> QSLVADVGDDHHAWHRLLDQALNQRRFELFFQPVVAAQDTQLVLHYKVLSRLLDEQGQTIPAGRFLPWLERFGWTARLDRLMLERV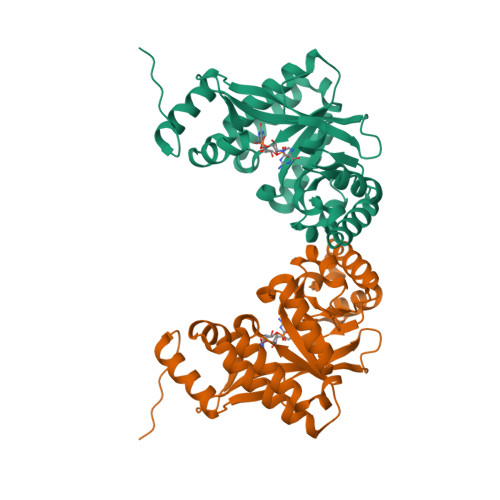LEQMAGHEESLALNLSSATLADPQALNKVFEILRAHSNLGARLTLEIGEEQLPEQAVLEQLTRRLRELGFSLSLQRFGGRFSMIGNLARLGLAYLKIDGSYIRAIDQESDKRLFIEAIQRAAHSIDLPLIAERVETEGELSVIREMGLYGVQGQLFGEPKPWG>[4x]SREDL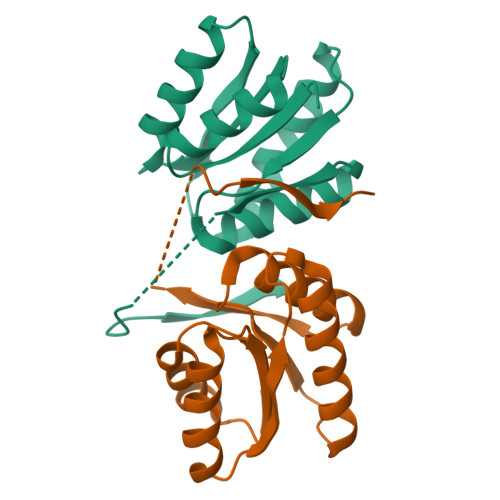RAWLTRNRFPRVGGVSESTVQWEGVVFTVSNESVPRWVMAQIQPAYMGLVATQASLAAAEAVAAVARRRGIEVHGPLQVADPNDPAASRSQVALLLSELRRAGCREIAVDLTGGKLPMSLGAFMAAEEAGVASLYVATDFDKHLKVPDMRTATLRQISQPE>MNNMNVIIADDHPIVLFGIRKSLEQIEWVNVVGEFEDSTALINNLPKLDAHVLITDLSMPGDKYGDGITLIKYIKRHFPSLSIIVLTMNNNPAILSAVLDLDIEGIVLKQGAPTDLPKALAALQKGKKFTPESVSRLLEKISAGGYGDKRLSPKESEVLRLFAEGFLVTEIAKKLNRSIKTISSQKKSAMMKLGVENDIALLNYLSSVTLSP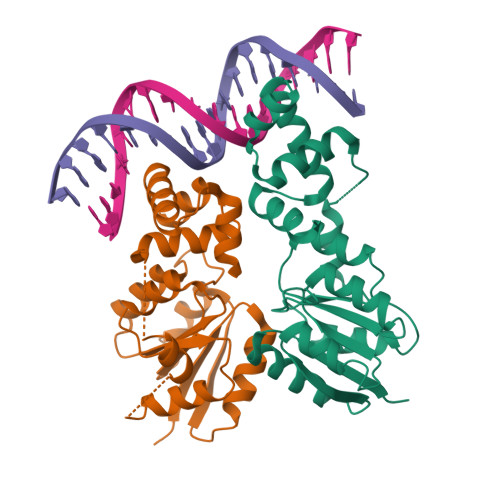ADKD[4x]>GPGSEFELRRQGNQDTYETHLETCRFEGLKEFLQQTDDRFHEMHVALAQKDQEIAFLRSMLGKLSEKIDQLEKSLE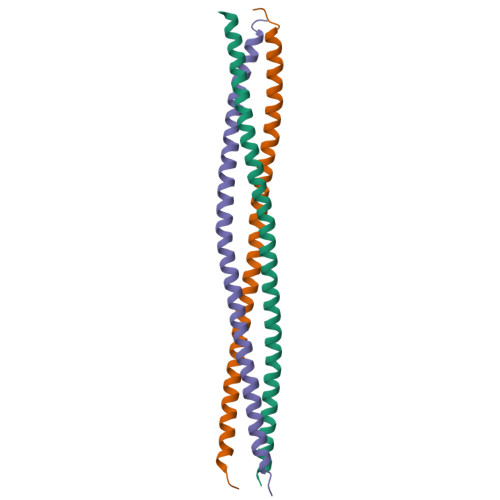LKFDVLDENQSKLSEDLMEFRRDASMLNDELSHINARLNMGILGS[3x]>MRFSREALLELEASRLAPYAQKARDTRGRAHPEPESLYRTPYQKDRDRILHTTAFRRLEYKTQVLPGWAGDYYRTRLTHTLEVAQVSRSIARALGLNEDLTEAIALSHDLGHPPFGHTGEHVLNALMQDHGGFEHNAQALRILTHLEVRYPGFRGLNLTYEVLEGI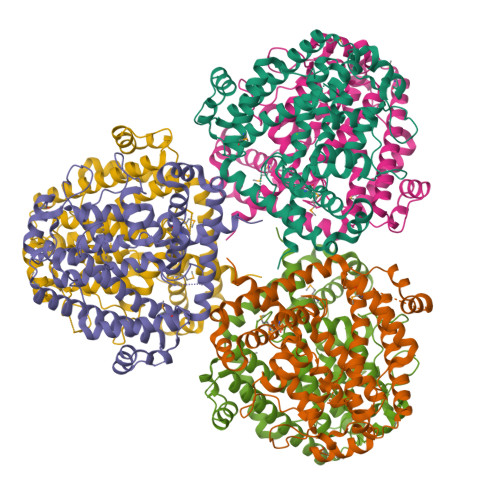ATHEAAYSPGFKPLYEGQGTLEAQVVDLSDAIAYAAHDLDDGFRAGLLHPEELKEVELLQALALEEGLDLLRLPELDRRVLVRQLLGYFITAAIEATHRRVEEAGVQSAEAVRRHPSRLAALGEEAEKALKALKAFLMERFYRHPEVLRERRKAEAVLEGLFAAYTRYPELLPREVQAKIPEEGLERAVCDYIAGMTDRFALEAYRRLSP[6x]> MGLEKTVKEKLSFEGVGIHTGEYSKLIIHPEKEGTGIRFFKNGVYIPARHEFVVHTNHSTDLGFKGQRIKTVEHILSVLHLLEITNVTIEVIGNEIPILDGSGWEFYEAIRKNILNQNREIDYFVVEEPIIVEDEGRLIKAEPSDTLEVTYEGEFKNFLGRQKFTFVEGNEEEIVLARTFAFDWEIEHIKKVGLGKGGSLKNTLVLGKDKVYNPEGLRYENEPVRHKVFDLIGDLYLLGSPVKGKFYSFRGGHSLNVKLVKELAKKQKLTRDLPH

Here, we describe our discovery and characterization of a biphenylacetylene-based inhibitor of LpxC, an essential enzyme in the biosynthesis of the lipid A component of the outer membrane of Gram-negative bacteria. Twenty years ago, the results of a study by Onishi and coworkers suggested that inhibition of LpxC, an essential cytoplasmic enzyme in the biosynthesis of lipid A in Gram-negative bacteria, was a promising strategy for countering Gram-negative bacterial infections. In view of LpxC’s key role in the biosynthesis of lipid A required for integrity of the outer membrane, the testing of LpxC inhibitors has revealed potent in vitro antibiotic activity against a broad spectrum of Gram-negative bacilli—including those harboring mobile carbapenemase-encoding resistance genes. The compound LPC-069 has no known adverse effects in mice and is effective in vitro against a broad panel of Gram-negative clinical isolates, including several multiresistant and extremely drug-resistant strains involved in nosocomial infections.

In order to visualize the mode of binding of LPC-069 to LpxC and to compare it with that of the previously studied inhibitor LPC-058 (14), we determined LPC-069’s crystal structure in a complex with Aquifex aeolicus LpxC, which is used as a model of Y. pestis LpxC. In the inhibitor-bound structure, LPC-069’s curved tail group occupies LpxC’s L-shaped hydrophobic substrate passage, and the terminal morpholine group adopts a chair conformation. Interestingly, the crystal structure featured two different head group conformations for LPC-069. In the major conformational state, the Cβ-substituted methyl group of the head group interacts with a conserved phenylalanine (F180) on LpxC, the hydroxyl group points toward the solvent, and the difluoromethyl moiety interacts with the conserved, catalytically important lysine (K227) and histidine (H253) residues in the active site. This type of interaction is consistent with that reported for LPC-058 (14). In the minor conformational state, however, the presence of a phosphate molecule in the active site causes LPC-069’s head group to undergo an ~120° rotation around its Cα-Cβ axis and thus distance itself from the protein’s residues. Given the very high phosphate concentration (~1.25 M) in the crystallization buffer, the minor conformation is probably a cocrystallization artifact rather than a bona fide binding mode. Compared with the major conformational state (in gray), the presence of a phosphate molecule in the minor conformational state (i) pushed the difluoromethyl group away from its energetically favorable position, (ii) caused an ~120° rotation around the head group’s Cα-Cβ bond, and (iii) disrupted the electrostatic interactions between the fluorine atoms and K227/H253.>[2x]MSK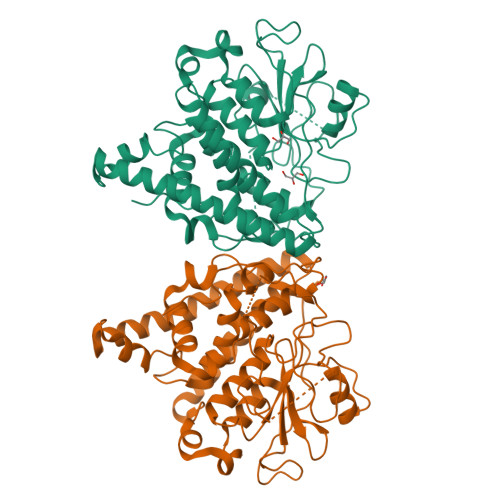QWASGTNGAFKRQVSSFRETISKQHPIYKPAKGRYWLYVSLACPWAHRTLITRALKGLTSVIGCSVVHWHLDEKGWRFLDMEKQLEDSEDFLEHWHDVAGGIRTAKEDSSKSFAEIKNDSQRFMVDATNEPHYGYKRISDLYYKSDPQYSARFTVPVLWDLETQTIVNNESSEIIRILNSSAFDEFVDDDHKKTDLVPAQLKTQIDDFNSWVYDSINNGVYKTGFAEKAEVYESEVNNVFEHLDKVEKILSDKYSKLKAKYGEEDRQKILGEFFTVGDQLTEADIRLYTTVIRFDPVYVQHFKCNFTSIRAGYPFIHLWVRNLYWNYDAFRYTTDFDHIKLHYTRSHTRINPLGITPLGPKPDIRPLLEHHHHHH1-Methyl-L-tryptophan 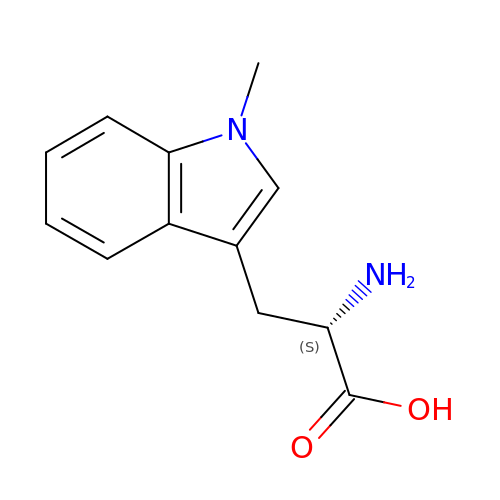| C12 H14 N2 O2 | ZADWXFSZEAPBJS-JTQLQIEISA-N> GMDDDQVAFSFILDNIVTQKMMAVPDSWPFHHPVNKKFVPDYYKVIVNPMDLETI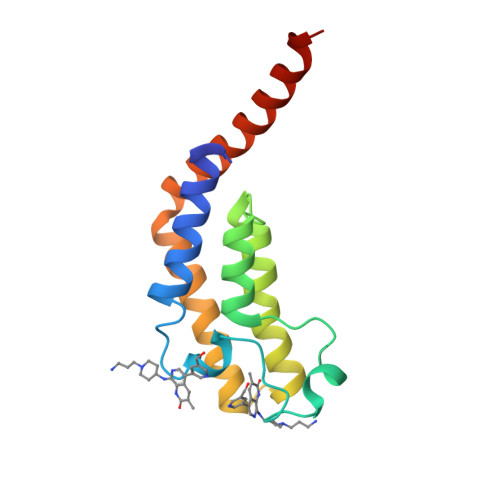RKNISKHKYQSRESFLDDVNLILANSVKYNGPESQYTKTAQEIVNVCYQTLTEYDEHLTQLEKDICTAKEAALEEAELESLD(1~{R},3~{R})-5-[(2~{E})-2-[(4~{a}~{R},5~{S},9~{a}~{S})-4~{a}-methyl-5-[(2~{R})-6-methyl-6-oxidanyl-heptan-2-yl]-3,4,5,6,7,8,9,9~{a}-octahydro-2~{H}-benzo[7]annulen-1-ylidene]ethylidene]cyclohexane-1,3-diol 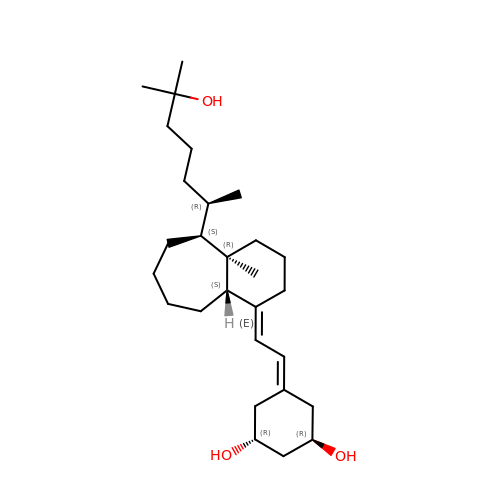| C28 H48 O3 | XEWIJHYWJALCQQ-UBGSZRSCSA-N> GAMGQEDEDGDYEELVLALRSEEDGLAEAPEHGTTATFHRCAKDPWRLPGTYVVVLKEETHLSQSERTARRLQAQAARRGYLTKILHVFHGLLPGFLVKMSGDLLELALKLPHVDYIEEDSSVFAQ;> SIPWNLERITPPRYRADEYQPPDGGSLVEVYLLDTSIQSDHREIEGRVMVTDFENVPEEDGTRFHRQASKCDSHGTHLAGVVSGRDAGVAKGASMRSLRVLNCQGKGTVSGTLIGLEFIRKSQLVQPVGPLVVLLPLAGGYSRVLNAACQRLARAGVVLVTAAGNFRDDACLYSPASAPEVITVGATNAQDQPVTLGTLGTNFGRCVDLFAPGEDIIGASSDCSTCFVSQSGTSQAAAHVAGIAAMMLSAEPELTLAELRQRLIHFSAKDVINEAWFPEDQRVLTPNLVAALPPSTHGAGWQLFCRTVWSAHSGPTRMATAVARCAPDEELLSCSSFSRSGKRRGERMEAQGGKLVCRAHNAFGGEGVYAIARCCLLPQANCSVHTAPPAEASMGTRVHCHQQGHVLTGCSSHWEVEDLGTHKPPVLRPRGQPNQCVG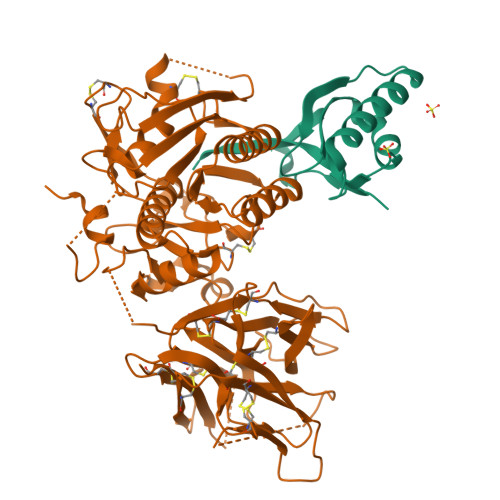HREASIHASCCHAPGLECKVKEHGIPAPQEQVTVACEEGWTLTGCSALPGTSHVLGAYAVDNTCVVRSRDVSTTGSTSEGAVTAVAICCRSRHLAQASQELQ>GSHMLFDFENDQVPSNIHFLNARASIETYTGINGEPSKGLKLAMQSKQHSYTGLAIVPEQPWDWSEFTSASLYFDIVSVGDHSTQFYLDVTDQNGAVFTRSIDIPVGKMQSYYAKLSGHDLEVPDSGDVNDLNLASGLRSNPPTWTSDDRQFVWMWGVKNLDLSGIAKISLSVQSAMHDKTVIIDNIRIQPNPPQDENFLVGLVDEFGQNAKVDYKGKI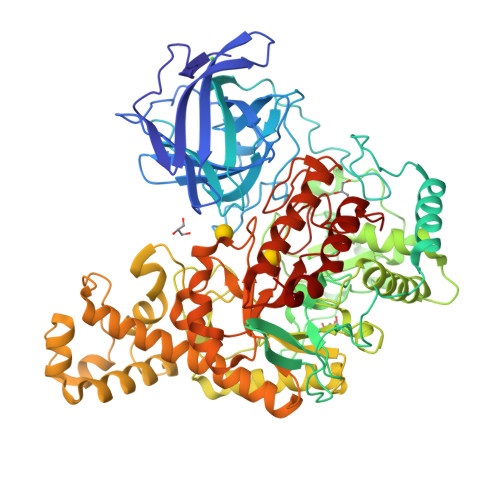HSLEELHAARDVELAELDGKPMPSRSKFGGWLAGPKLKATGYFRTEKINGKWMLVDPEGYPYFATGLDIIRLSNSSTMTGYDYDQATVAQRSADDVTPEDSKGLMAVSEKSFATRHLASPTRAAMFNWLPDYDHPLANHYNYRRSAHSGPLKRGEAYSFYSANLERKYGETYPGSYLDKWREVTVDRMLNWGFTSLGNWTDPAYYDNNRIPFFANGWVIGDFKTVSSGADFWGAMPDVFDPEFKVRAMETARVVSEEIKNSPWCVGVFIDNQKSFGRPDSDKAQYGIPIHTLGRPSEGVPTRQAFSKLLKAKYKTIAALNNAWGLKLSSWAEFDLGVDVKALPVTDTLRADYSMLLSAYADQYFKVVHGAVEHYMPNHLYLGARFPDWGMPMEVVKAAAKYADVVSYNSYKEGLPKQKWAFLAELDKPSIIGEFHIGAMDHGSYHPGLIHAASQADRGEMYKDYMQSVIDNPYFVGAHWFQYMDSPLTGRAYDGENYNVGFVDVTDTPYQEMVDAAKEVNAKIYTERLGSK[2x]(2~{S})-2-[[(2~{S})-6-[[(2~{S})-2-[[4-[[[(2~{S})-2-[[(2~{R})-2-[(6-fluoranylpyridin-3-yl)carbonylamino]-3-sulfo-propanoyl]amino]-3-sulfo-propanoyl]amino]methyl]phenyl]carbonylamino]-3-naphthalen-2-yl-propanoyl]amino]-1-oxidanyl-1-oxidanylidene-hexan-2-yl]carbamoylamino]pentanedioic 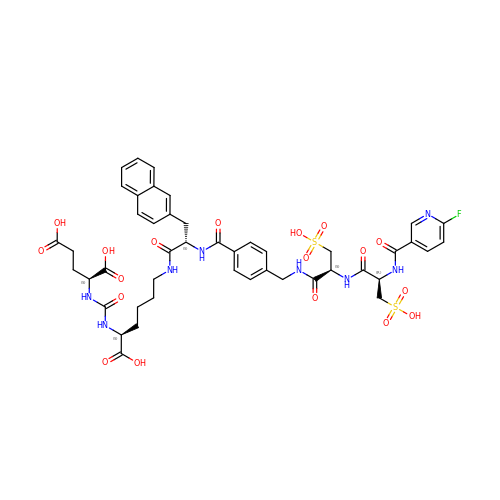acid | C45 H51 F N8 O18 S2 | FRBOTEDIQNCFCM-ISWDJSIVSA-N>GAMGSGSSLSPTEGKGSGLQGHIIENPQYFSDACVHHIKRRDIVLKWELGEGAFGKVFLAECHNLLPEQDKMLVAVKALKEASESARQDFQREAELLTMLQHQHIVRFFGVCTEGRPLLMVFEYMRHGDLNRFLRSHGPDAKLLAGGEDVAPGPLGLGQLLAVASQVAAGMVYLAGLHFVHRDLATRNCLVGQGLVVKIGDFGMSRDIYSTDYYRVGGRTMLPIRWMPPESILYRKFTTESDVWSFGVVLWEIFTYGKQPWYQLSN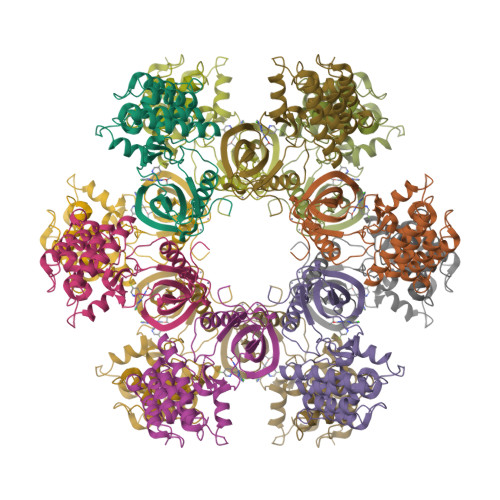TEAIDCITQGRELERPRACPPEVYAIMRGCWQREPQQRHSIKDVHARLQALAQAPPVYLDVLG[3x]>[2x]GSHMRKQQRMVVVRAEGGGGINPEIRKN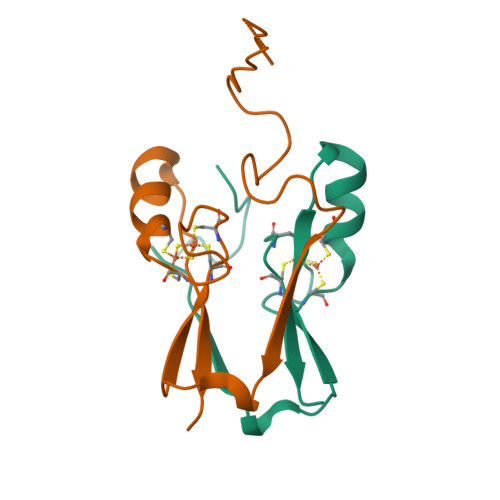EDKVVDSVVVTELSKNITPYCRCWRSGTFPLCDGSCVKHNKANGDNVGPLLLKKQ>[4x]MAHHHHHHMSTSSRCLVRGSVNIDEFFHLPHIVRPGETISSTGLTKRAGGKGAN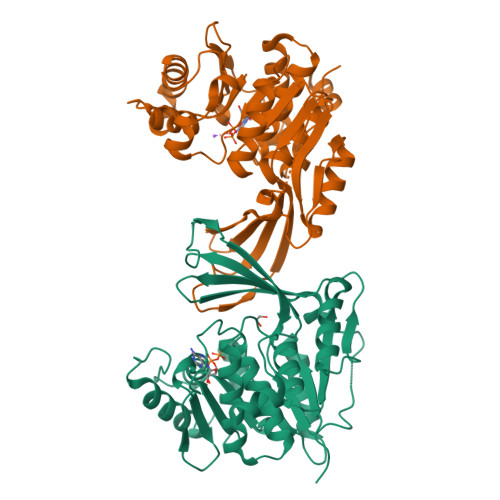QAFAVARAGGQVELDGAIGDDGIWVKEMLESAGVGTDKLKIVKDEVTGRAVIQSAADGENSIVLHAGANYYLPSPTPTTSLATYTHLLVQNEVPLSSTLAYLTAAGQSSPPLTSVFNPSPMLTPAQLREFPWKHLSWLIVNEGELGDLLLAFGSSANPGEAKEDELQAKASAGILELHENDYFSKNVGIICTLGAKGILCYEPGKEVGYLPAAKLQNPVKDTTGAGDCFAGYFVAGLMSGKSLQDALKTCLVACGICVENEGAMESVPTLNAVKERLA>MQKAVEITYNGKTLRGMMHLPDDVKGKVPMVIMFHGFTGNKVESHFIFVKMSRALEKVGIGSVRFDFYGSGESDGDFSEMTFSSELEDARQILKFVKEQPTTDPERIGLLGLSMGGAIAGIVAREYKDEIKALVLWAPAFNMPELIMNESVKQYGAIMEQLGFVDIGGHKLSKDFVEDISKLNIFELSKGYDKKVLIVHGTNDEAVEYKVSDRILKEVYGDNATRVTIENADHTFKSLEWEKKAIEESVEFFKKELLKG[2x]

Lipases are enzymes that reversibly catalyze the hydrolysis and synthesis of a large variety of glycerol esters. A minimal lid domain comprising the residues 141-183 is inserted between strand β6 and helix αE on top of the CD active-site area. Different from most other lipases, in which the lid is generally formed by a bundle of α-helices, in Tth MAG lipase this domain is compact. It is formed by two small α-helices, followed by a β-hairpin and an additional α-helix, referred to as α-helix/β-hairpin/α-helix (HBH).

Next, we determined its high-resolution crystal structure, both in the presence and absence of the covalent active site serine protease inhibitor phenylmethylsulfonyl fluoride (PMSF). In the active site of both Tth MAG lipase structures, with and without PMSF, we observed literally identical density of a glycerol molecule, presenting one of the two final products of esterase/lipase catalysis. The glycerol molecule tightly interacts via its two C2 and C3 hydroxyl groups with the carboxylate group of a non-conserved active-site residue Glu43, specific to Tth MAG lipase. In the presence of the C18 MAG reaction intermediate, there are significant alterations in the packing arrangement of several residues within the lid core when comparing to the PMSF-inhibited structure. The largest spatial deviations are found in the N-terminal part of the lid domain, which includes the first two lid helices α-LA and α-LB. In the Tth MAG lipase ternary complex structure these two helices are separated by a short loop, whereas in the PMSF-inhibited structure both merge into one long helix (residues 142–161) with a sharp kink at residue Gln153. As a result, in the PMSF-inhibited structure the side chains of Ser150 and Tyr154 next to the kink block the formation of the lid tunnel.> EKQLMNVEPIHADILLETYKRKIADEGRPFLAEFQSIPRVFSKFPIKEARKPFNQNKNRYVDILPYDYNRVELSEINGDAGSNYINASYIDGFKEPRKYIAAQGPRDETVDDFWRMIWEQKATVIVMVTRCEEGNRNKCAEYWPSMEEGTRAFGDVVVKINQHKRCPDYIIQKLNIVNKKEKATGREVTHIQFTSWPDHGVPEDPHLLLKLRRRVNAFSNFFSGPIVVHSSAGVGRTGTYIGIDAMLEGLEAENKVDVYGYVVKLRRQRCLMVQVEAQYILIHQALVEYNQFGETEVNLSELHPYLHNMKKRDPPSEPSPLEAEFQRLPSYRSWRTQHIGNQEENKSKNRNSNVIPYDYNRVPLKHELEMSKESEHDSDESSDDDSDSEEPSKYINASFIMSYWKPEVMIAAQGPLKETIGDFWQMIFQRKVKVIVMLTELKHGDQEICAQYWGEGKQTYGD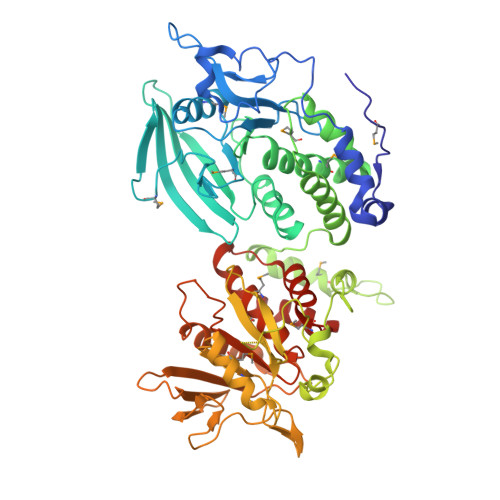IEVDLKDTDKSSTYTLRVFELRHSKRKDSRTVYQYQYTNWSVEQLPAEPKELISMIQVVKQKLPQKNSSEGNKHHKSTPLLIHCRDGSQQTGIFCALLNLLESAETEEVVDIFQVVKALRKARLGMVSTFEQYQFLYDVIASTYPAQN>[4x]GMGTVSKALTLLTYFNHGRLEIGLSDLTRLSGMNKATVYRLMSELQEAGFVEQVEGARSYRLGPQVLRLAALREASVPILSASRRVLRELSEDTGETTHLSLLQGEQLASLSHAYSSRNATKVMMEDAEVLTFHGTASGLAVLAYSEPSFVD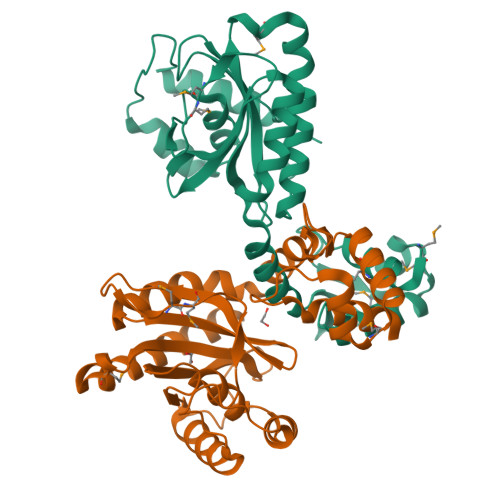AVLAAPLTARTPQTQTDPAAIRAEIAEVRRTGLAQSIGGFEAEVHSHAVPIFGPDRAVLGALAVAAPTSRMTPDQKRTIPPALRAAGLSLTERIGGACPPEFPTDIAA ISATOIC ANHYDRIDE | C7 H9 N O | 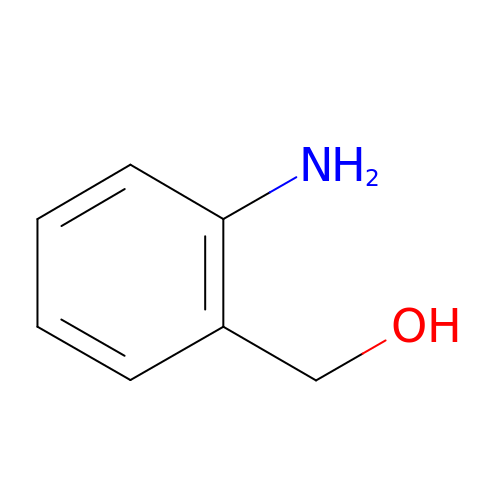VYFOAVADNIHPTR-UHFFFAOYSA-N> SLRFTASTSTPKSGSKIAKRGKKHPEPVASWMSEQRWAGEPEVMCTLQHKSIAQEAYKNYTITTSAVCKLVRQLQQQALSLQVHFERSER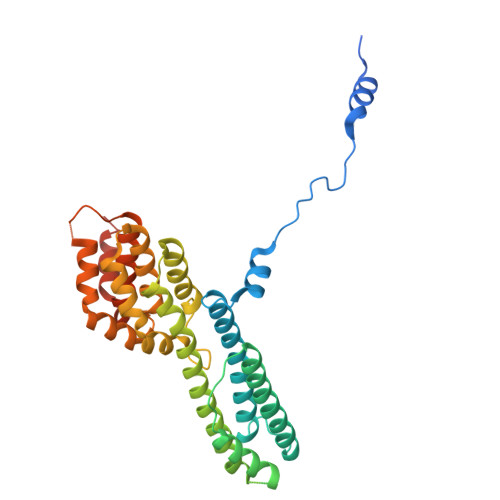VLSGLQASSLPEALAGATQLLSHLDDFTATLERRGVFFNDAKIERRRYEQHLEQIRTVSKDTRYSLERQHYINLESLLDDVQLLKRHTLITLRLIFERLVRVLVISIEQSQCDLLLRANINMVATLMNIDYDGFRSLSDAFVQNEAVRTLLVVVLDHKQSSVRALALRALATLCCAPQAINQLGSCGGIEIVRDILQVESAGERGAIERREAVSLLAQITAAWHGSEHRVPGLRDCAESLVAGLAALLQPE>PPRGKTVWFTGLSGSGKSSVAMLVERKLLEKGISAYVLDGDNLRHGLNADLGFSMADRAENLRRLSHVATLLADCGHLVLVPAISPLAEHRALARKVHADAGIDFFEVFCDTPLQDCERRDPKGLYAKARAGEITHFTGIDSPYQRPKNPDLRLTP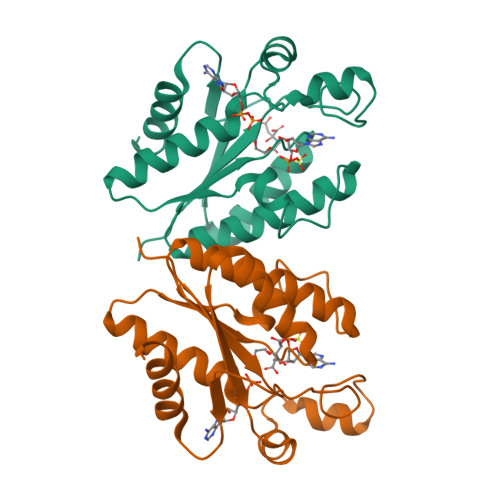DRSIDEQAQEVIDLLES[2x]>DKWEMERTDITMKHKLGGGQYGEVYEGVWKKYSLTVAVKTLKEDTMEVEEFLKEAAVMKEIKHPNLVQLLGVCTREP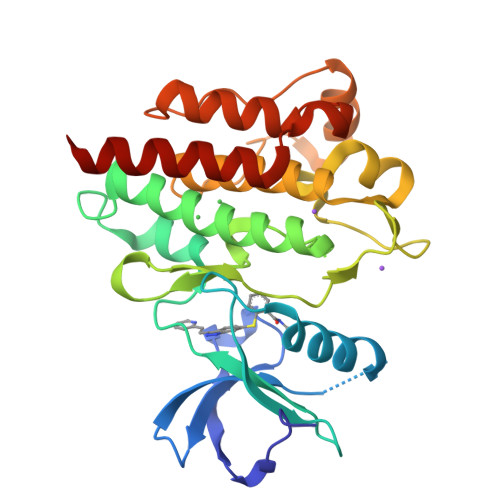PFYIIIEFMTYGNLLDYLRECNRQEVNAVVLLYMATQISSAMEYLEKKNFIHRDLAARNCLVGENHLVKVADFGLSRLMTGDTYTAHAGAKFPIKWTAPESLAYNKFSIKSDVWAFGVLLWEIATYGMSPYPGIDLSQVYELLEKDYRMERPEGCPEKVYELMRACWQWNPSDRPSFAEIHQAFETMFQESSIS[2x]> SNAVRIEITQGVDSARPIGVVPFKWAGPGAAPEDIGGIVAADLRNSGKFNPLDRSRLPQQPATAQEVQPTAWSALGIDAVVVGQVTPNPDGSYNVAYQLVDTGGAPGTVLAQNSYKVNKQWLRYAGHTASDEVFEKLTGIKGAFRTRIAYVVQTNGGQFPYELRVSDYDGYNQFVVHRSPQPLMSPAWSPDGSKLAYVTFESGRSALVIQTLANGAVRQVASFPRHNGAPAFSPDGTKLAFALSKTGSLNLYVMDLASGQIRQITDGRSNNTEPTWFPDSQTLAFTSDQAGRPQVYKMNINGGAAQRITWEGS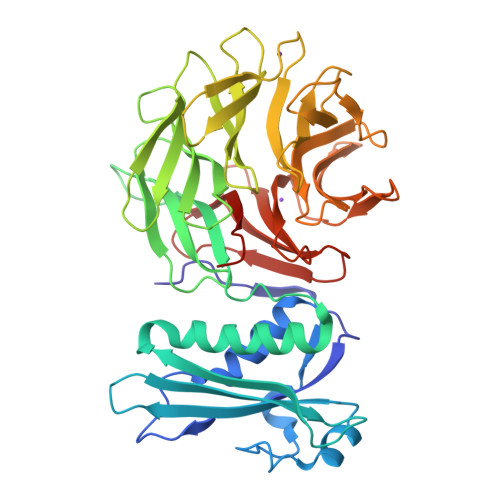QNQDADVSSDGKFMVMVSSNNGQQHIAKQDLVTGGVQVLSSTFLDETPSLAPNGTMVIYSSSQGMGSVLNLVSTDGRFKARLPATDGQVKSPAWSPYL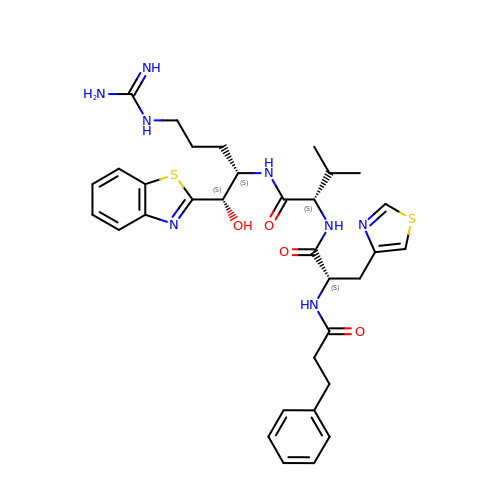N-(3-phenylpropanoyl)-3-(1,3-thiazol-4-yl)-L-alanyl-N-[(1S,2S)-1-(1,3-benzothiazol-2-yl)-5-carbamimidamido-1-hydroxypentan-2-yl]-L-valinamide | C33 H42 N8 O4 S2 | AHZGKBJWEMYHLE-NSIYGSDQSA-N> ANVWGVRLADSLSSPTIETRTRQYTLHDLCSDLDANPGREPWKPLRNQRTNNIVAVQLFRPLQGLVLDTQLYGFPGAFDDWERFMREKLRVLKYEVLRIYPISNYSNEHVNVFVANALVGAFLSNQAFYDLLPLLIINDTMIGDLLGTGASLSQFFQSHGDVLEVAAGRKYLQMENYSNDDDDPPLFAKDLSDYAKAFYSDTYEVLDRFFWTHDSSAGVLVHYDKPTNGHHYLLGTLTQMVSAPPYIINATDAMLLESCLEQFSANVRARPAQPVTRLDQCYHLRWGAQYVGEDSLTYRLGVLSLLATNGYQLARPIPRQLTNRWLSSFVSQIMSDGVNETPLWPQERYVQIAYDSPSVVDGATQYGYVRKNQLRLGMRISALQSLSDTPSPVQWLPQYTIDQAAMDEGDLMVSRLTQLPLRPDYGNIWVGDALSYYVDYNRSHRVVLSSELPQLPDTYFDGDEQYGRSLFSLARKIGDRSLVKDTAVLKHAYQAIDPNTGKEYLRSRQSVAYFGASAGHSGADQPLVIEPWIQGKISGVPPPSSVRQFGYDVARGAIVDLARPFPSGDYQFVYSDVDQVVDGHDDLSISSGLVESLLSSCMHATAPGGSFVVKINFPTRPVWHYIEQKILPNITSYMLIKPFVTNNVELFFVAFGVHQHSSLTWTSGVYFFLVDHFYRYETLSTISRQLPSFGYVDDGSSVTGIETISIENPGFSNMTQAARIGISGLCANVGNARKSIAIYESHGARVLTITSRRSPASARRKSRLRYLPLIDPRSLEVQARTILPADPVLFENVSGASPHVCLTMMYNFEVSSAVYDGDVVLDLGTGPEAKILELIPATSPVTCVDIRPTAQPSGCWNVRTTFLELDYLSDGWITGVRGDIVTCMLSLGAAAAGKSMTFDAAFQQLIKVLSKST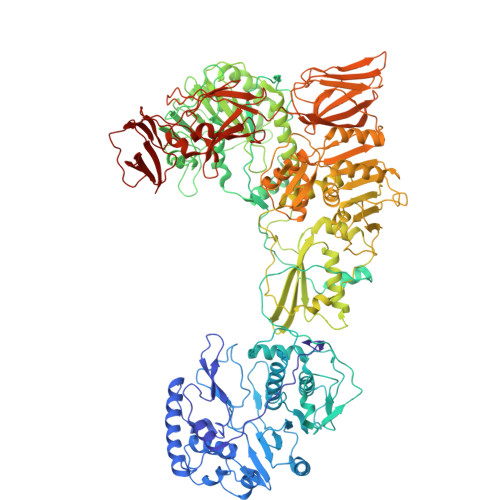ANVVLVQVNCPTDVVRSIKGYLEIDSTNKRYRFPKFGRDEPYSDMDALEKICRTAWPNCSITWVPLSYDLRWTRLALLESTTLSSASIRIAELMYKYMPIMRIDIHGLPMEKRGNFIVGQNCSLVIPGFNAQDVFNCYFNSALAFSTEDVNAAMIPQVSAQFDATKGEWTLDMVFSDAGIYTMQALVGSNANPVSLGSFVVDSPDVDITDAWPAQLDFTIAGTDVDITVNPYYRLMTFVRIDGQWQIANPDKFQFFSTLVMNVKLDIADKYLLYYIRDVQSRDVGFYIQHPLQLLNTITLPTNEDLFLSAPDMREWAVKESGNTICILNSQGFVLPQDWDVLTDTISWSPSIPTYIVPPGDYTLTPL>[2x]MVSFRLSGATSSSYGVFISNLRKALPNERKLYDIPLLRSSLPGSQRYALIHLTNYADETISVAIDVTNVYIMGYRAGD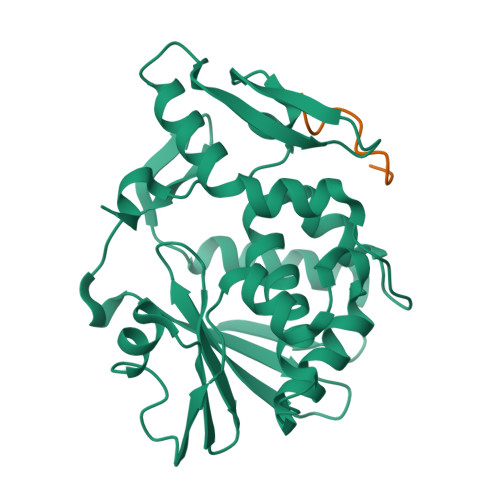TSYFFNEASATEAAKYVFKDAMRKVTLPYSGNYERLQTAAGKIRENIPLGLPALDSAITTLFYYNANSAASALMVLIQSTSEAARYKFIEQQIGKRVDKTFLPSLAIISLENSWSALSKQIQIASTNNGQFESPVVLINAQNQRVTITNVDAGVVTSNIALLLNRNNMA;>SDDDMGFGLFD[2x]> MRNEMHLQFSARSENESFARVTVAAFVAQLDPTMDELTEIKTVVSEAVTNAIIHGYNNDPNGIVSISVIIEDGVVHLTVRDEGVGIPDIEEARQP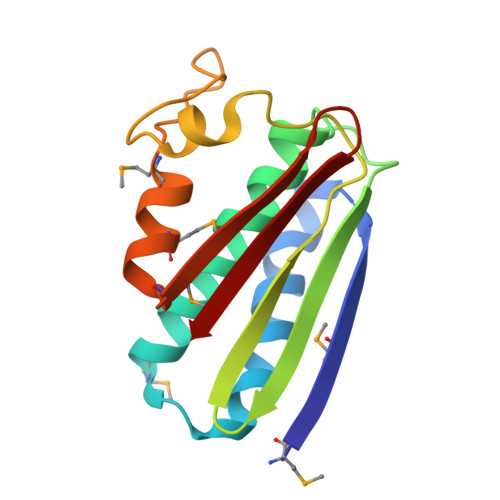LFTTKPELERSGMGFTIMENFMDEVIVESEVNKGTTVYLKK>[2x]MKHDYTNPPWNAKVPVQRAMQWMPISQKAGAAWGVDPQLITAIIAIESGGNPNAVSKSNAIGLMQLKASTSG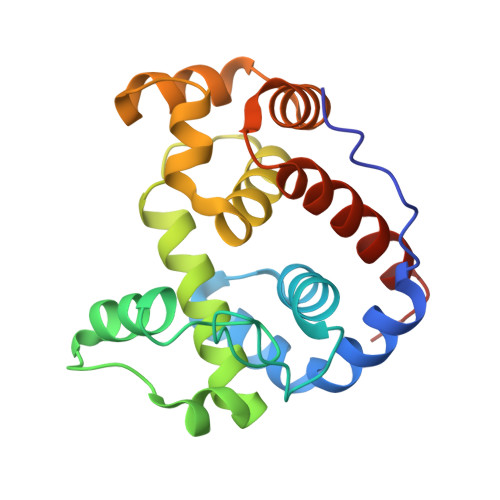RDVYRRMGWSGEPTTSELKNPERNISMGAAYLNILETGPLAGIEDPKVLQYALVVSYANGAGALLRTFSSDRKKAISKINDLDADEFLEHVARNHPAPQAPRYIYKLEQALDAMLEHHHHHH> MSFFRDLLESVVPTAYAEEPVEDVEVEQPEDAPEEEVSEETVEEEEEDDEDDDEDDEEEEETADPLDTLREECTKTAACKPFDHHFHECIERVTKEQEEPDYEHKHYKEDCIEEFFHLQHCVNDCVAPRLFN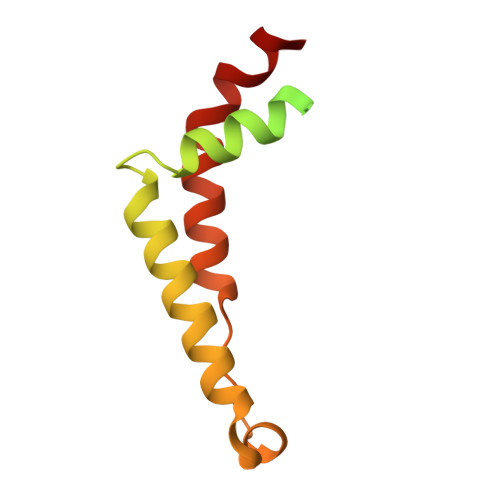RLK(2R)-N,2,7-trimethyl-2,3-dihydro-4H-1,4-benzoxazine-4-carboxamide | C12 H16 N2 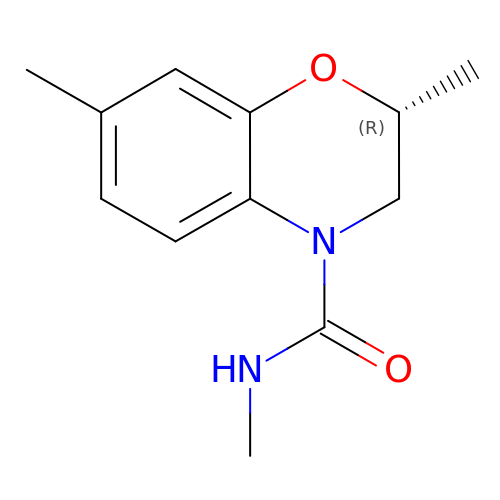O2 | FWSAWLIRIYMUOD-SECBINFHSA-N Here we demonstrate that CEP85 is essential for faithful centriole duplication through a direct interaction with the previously uncharacterised N-terminal domain of STIL, a key factor involved in the early steps of centriole formation. Subsequently, through its C-terminal PB3, PLK4 interacts with STIL and phosphorylates it, enabling STIL to recruit SASS6 to the site of procentriole assembly.

Subsequently, we also determined the structure of the complex between Trichoplax adhaerens STIL-NTD and human CEP85 cc4 by X-ray crystallography to a resolution of 4.6 Å. The structure of the complex was solved by MAD using crystals of the corresponding selenomethionine derivative. The structure of the CEP85-STIL complex shows a 2:2 binding ratio with one STIL NTD bound to each of the two coiled-coil strands of the parallel CEP85 cc4 dimer. Compared with the unbound CEP85 coiled-coil structure we did not observe any density for the N-terminal half of the coiled-coil, probably due to its partial unfolding in the crystal. The interaction between the CEP85 coiled-coil and STIL NTD involves mainly subdomain 1 of STIL, in particular the region of the β-barrel capping helix and the crossover hairpin-loop that, together, constitute one of the two conserved patches in the STIL NTD. Each of the STIL NTDs interacts with both CEP85 coiled-coil helices. The crossover hairpin-loop of subdomain 1 of STIL NTD contacts towards the N-terminal part of one of the coiled-coil helices, whereas its barrel capping helix contacts towards the C-terminal end of the other CEP85 coiled-coil helix. Due to the relatively low resolution of the complex structure we could not resolve any sidechains. However, several conserved residues of the CEP85 coiled-coil and STIL subdomain 1 would be well placed to make electrostatic and hydrophobic interactions with each other. The structure of the complex between STIL NTD and CEP85 cc4 indicated that the highly conserved residues L47 and R50 in Trichoplax adhaerens STIL (L64 and R67 in human STIL, L60 and R63 in Gallus gallus STIL) and human CEP85 Q640 and E644 are located at their interaction interface.

> GGSMATNENLPEIMTKLWDSKAQGEQEELHLLKGSDCNLTIDITEKCLRLAQRSAYQLHTETSATKRIQKFFLLGSLNINKDDRVIINIDRFDPGRIIDRKEGNKSLHVPTAVIPGDVIIPLSMQLACLGSEGVSPFSISEYYDAFQTLTKNLKLSCDSVDIKDMLSLKIHATYYVDSDEISINVTSGVVVPSALITAVPILPVSIVPTALARSLSGPLHLSNFQDTQKSGYVAINNSHNLLLVLDSDPKLSSIPLVGIWVDGVISIHHPYVWSACMRYLYSQRLTNKIRDGSTGFILVLYTQTRPKPEFWECSFSGKSDKFLYCQASDDIFMEKVAKTRNEYMRLQLVPNEFGENLYFQ;> GESWQKRYDSLQKIVEKQQQKMDQLRSQVQSLEQEVAQEEGTSQALREEAQRRDSALQQLRTAVKELSVQNQDLIEKNLTLQEHLRQA> MGSSHHHHHHSQDPMSLIKKKNKDIRIIPLGGVGEIAKNMYIVEVDDEMFMLDAGLMFPEDEMLGVDIVIPDIQYVIENKERLKGIFLTHGHEHAIGAVSYVLEQIDAPVYGSKLTIALVKEAMKARNIKKKVRYYTVNHDSIMRFKNVNVSFFNTTHSIPDSLGVCIHTSYGSIVYTGAFKFDQSLHGHYAPDLKRMAEIGDEGVFALISDSTEAEKPGYNTPENIIEH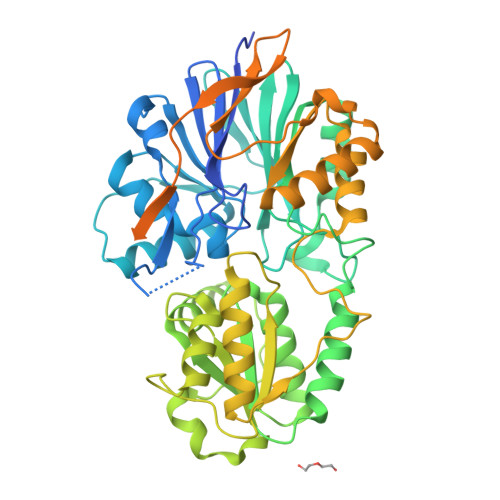HMYDAFAKVKGRLIVSCYASNFVRIQQVLNIASQLNRKVSFLGRSLESSFNIARKMGYFDIPKDLLIPINEVENYPKNEVIIIATGMQGEPVEALSQMARKKHKIMNIEEGDSIFLAITASANMEVIIADTLNELVRAGAHIIPNNKKIHASSHGCMEELKMMLNIMKPEYFVPVQGEFKMQIAHAKLAAETGVAPEKIFLVEKGDVISYNGKDMILNEKVQSGNILIDGIGVGDVGNIVLRDRHLLAEDGIFIAVVTLDPKNRRIAAGPEIQSRGFVYVRESEELLKEAEEKVRKIVEEGLQEKRIEWSEIKQNMRDQISKLLFESTKRRPMIIPVISEI>[4x]MRKTKTEALKTKEHLMLAALETFYRKGIARTSLNEIAQAAGVTRGALYWHFKNKEDLFDALFQRICDDIENCIAQDAADAEGGSWTVFRHTLLHFFERLQSN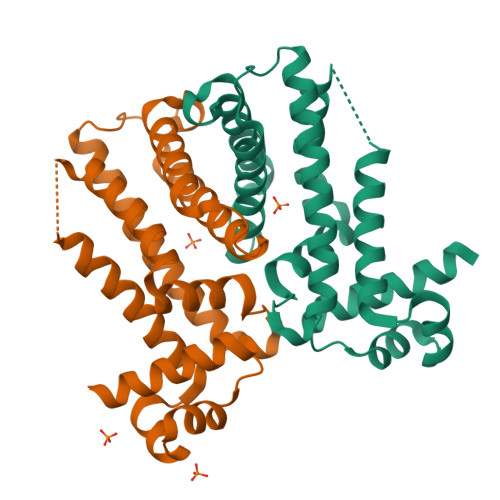DIHYKFHNILFLKCEHTEQNAAVIAIARKHQAIWREKITAVLTEAVENQDLADDLDKETAVIFIKSTLDGLIWRWFSSGESFDLGKTAPRIIGIMMDNLENHPCLRRK> GPHMPFTLASAQAIFAGVAPSRIPAILAEFNRLSIEDRLGLL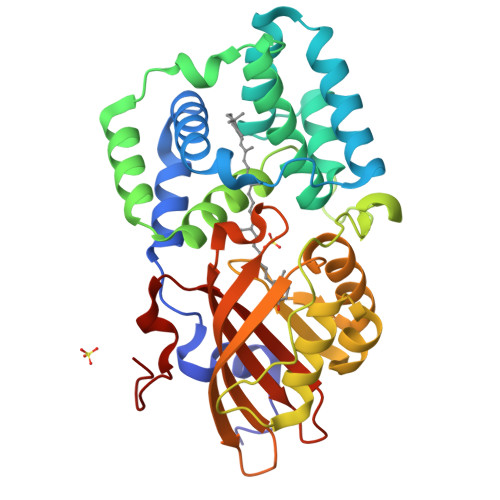WFAYTETGRSITRAALGAASMSLVENLLNEIKQKSRAEQTQVMIDIASRADTPISRSYGYFSANTKLGFWYQLAEWMAQGLVAPAPKDYQLSSAANDLFNTIKKLDGGQQIQVLRDIVVNMGFDASVAPAPAPKAEEFQFERTEPVVSGLKVDGINDPTPLAYFEAMNRDDFETAVNLFAEDGALQPPFQKPIVGREAILKYMREEAQGLNMRPAQGIAEVLPDGSKQLRVTGKVQTPWFGVNVAMNLAWRFALNPDGKIFFVAIDMLGSPEELLNLRPPSYR>[4x]XIEELLRKI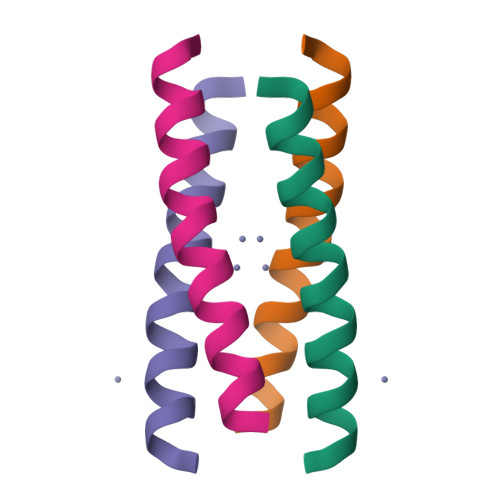IEDDVRHIAELEDIEKWLX> MGSSHHHHHHSSGLVPRGSHMPSASASRKSQEKPRE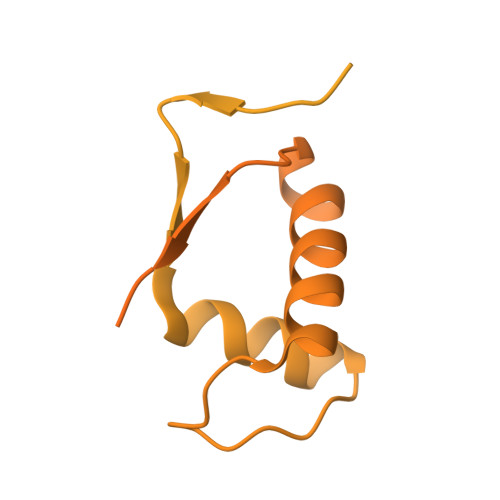IMDAAEDYAKERYGISSMIQSQEKPDRVLVRVRDLTIQKADEVVWVRARVHTSRAKGKQCFLVLRQQQFNVQALVAVGDHASKQMVKFAANINKESIVDVEGVVRKVNQKIGSCTQQDVELHVQKIYVISLAEPRLPLQLDDAVRPEAEGEEEGRATVNQDTRLDNRVIDLRTSTSQAVFRLQSGICHLFRETLINKGFVEIQTPKIISAASEGGANVFTVSYFKNNAYLAQSPQLYKQMCICADFEKVFSIGPVFRAEDSNTHRHLTEFVGLDIEMAFNYHYHEVMEEIADTMVQIFKGLQERFQTEIQTVNKQFPCEPFKFLEPTLRLEYCEALAMLREAGVEMGDEDDLSTPNEKLLGHLVKEKYDTDFYILDKYPLAVRPFYTMPDPRNPKQSNSYDMFMRGEEILSGAQRIHDPQLLTERALHHGIDLEKIKAYIDSFRFGAPPHAGGGIGLERVTMLFLGLHNVRQTSMFPRDPKRLTP> MGSSHHHHHHSQDPVHFYETSYKYQAADSTYMHDVAINVSIKGNHFTSDIIIRELVKSENKNYYNVIGHGDIIQKN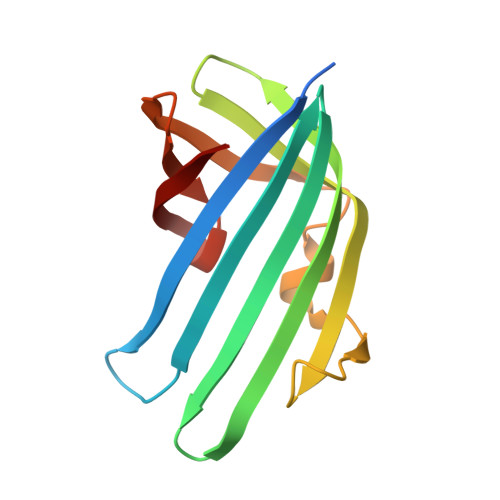THQYYLNFDNIDVYTGTNKANMKPYKEPTSISSLINKSNNIRVVYLSEEYVVVEFFFYDGQIITLHRY> MDQQSTRTDITVNVDGFWMLQALLDIRHVAPELRCRPYVSTDSNDWLNEHPGMAVMREQGIVVGDTVNEQVAARMRVLAAPDLEVVALLSRGKLLYGVVDNEDQPPGSRDIPDNEFRVVLARRGQHWVSAVRVGNDITV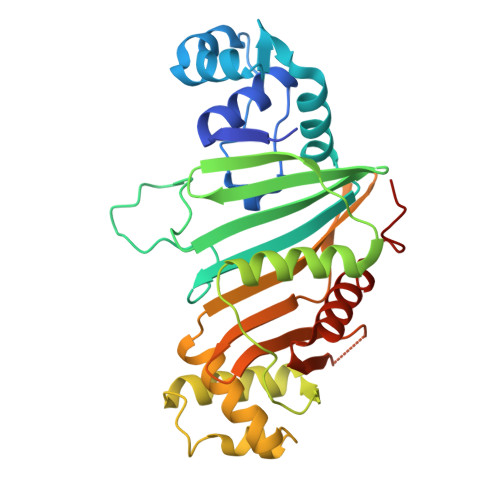DDVSVSDSASIAALVIDGLESIHHADPAAINAVNVPLEEMLEATKSWQESGFNVFSGGDLRRMGISASTVAALGQALSDPAAEVAVYARQYRDDAKGPSASVLSLKDGSGGRIALYQQARTAGSGEAWLAICPATPQLVQVGVKTVLDTLPYGEWKTHSRV4-(1H-1,2,4-triazol-1-yl)quinolin-6-amine | C11 H9 N5 | 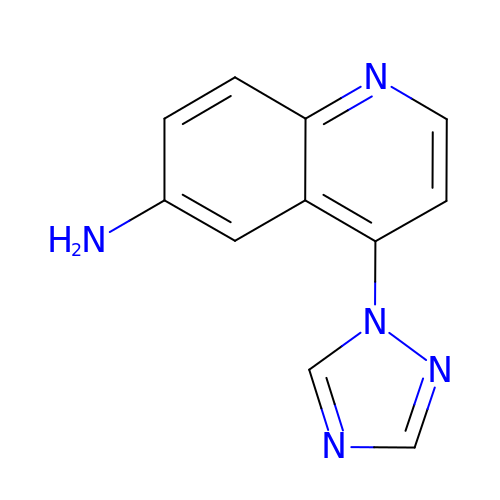GXRXDACPFFYIDQ-UHFFFAOYSA-N>AFAR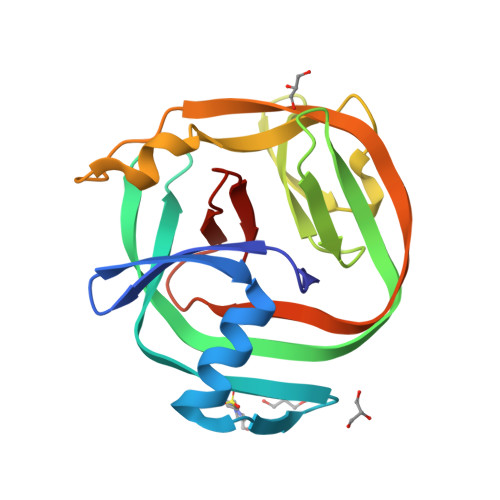DTEVYYENDTVPHMESIEEMYSKYASMNGELPFDNGYAVPLDNVFVYTLDIASGEIKKTRASYIYREKVEKLIEIKLSSGYSLKVTPSHPVLLFRDGLQWVPAAEVKPGDVVVGVREEVLRRRIISKGELEFHEVSSVRIIDYNNWVYDLVIPETHNFIAPNGLVLHNAQ[2x]>SIAAEREAALERPRRTKRERDQLYYECYSDVSVHEEMIADRVRTDAYRLGILRNWAALRGKTVLDVGAGTGILSIFCAQAGARRVYAVEASAIWQQAREVVRFNGLEDRVHVLPGPVETVELPEQVDAIVSEWMGYGLLHESMLSSVL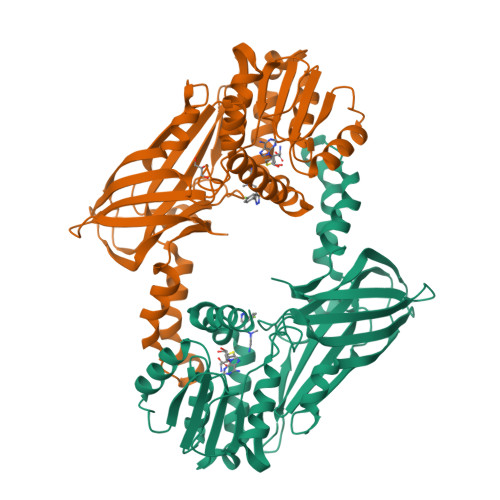HARTKWLKEGGLLLPASAELFIAPISDQMLEWRLGFWSQVKQHYGVDMSCLEGFATRCLMGHSEIVVQGLSGEDVLARPQRFAQLELSRAGLEQELEAGVGGRFRCSCYGSAPMHGFAIWFQVTFPGGESEKPLVLSTSPFHPATHWKQALLYLNEPVQVEQDTDVSGEITLLPSRDNPRRLRVLLRYKVGDQEEKTKDFAMED[2x]> MKPEIEQELSHTLLTELLAYQFASPVRWIETQDVFLKQHNTERIIEIGPSPTLAGMANRTIKAKYESYDAALSLQRQVLCYSKDAKEIYYKPDPADLAPKETPKQEESTPSAPAAATPTPAAAAAPTPAPAPASAGPVESSSGAGSGAGAANSGGAVVDSAALDALTAENKKLAKQQLEVLARYLQVDLNKGSAKSFIKEKEASAVLQKELDLWEAEHGEFYAKGIQPTFSALKSRTYDSYWNWARQDVLSMYFDIIFGKLTSVDRETINQCIQIMNRANPTLIKFMQYHIDHCPEYKGETYKLAKRLGQQLIDNCKQVLTEDPVYKDVSRITGPKTKVSAKGNIEYEETQKDSVRKFEQYVYEMAQGGAMTKVSQPTIQEDLARVYKAISKQASKDSKLELQRVYEDLLKVVESSKEIETEQLTKDILQAATVPTTPTEEVDDPCTPSSDDEIASLPDKTSIIQPVSSTIPSQTIPFLHIQKKTKDGWEYNKKLSSLYLDGLESAAINGLTFKDKYVLVTGAGAGSIGAEILQGLISGGAKVIVTTSRFSKKVTEYYQNMYARYGAAGSTLIVVPFNQGSKQDVDALVQYIYDEPKKGGLGWDLDAIIPFAAIPENGNGLDNIDSKSEFAHRIMLTNLLRLLGAVKSKKTTDTRPAQCILPLSPNHGTFGFDGLYSESKISLETLFNRWYSEDWGSKLTVCGAVIGWTRGTGLMSANNIIAEGIEKLGVRTFSQKEMAFNILGLLTPEIVQLCQEEPVMADLNGGLQFIDNLKDFTSKLRTDLLETADIRRAVSIESAIEQKVVNGDNVDANYSKVMVEPRANMKFDFPTLKSYDEIKQIAPELEGMLDLENVVVVTGFAEVGPWGNSRTRWEMEAYGEFSLEGAIEMAWIMGFIKYHNGNLKGKPYSGWVDAKTQTPIDEKDIKSKYEEEILEHSGIRLIEPELFNGYDPKKKQMIQEVVVQHDLEPFECSKETAEQYKHEHGEKCEIFEIEESGEYTVRILKGATLYVPKALRFDRLVAGQIPTGWDARTYGIPEDTISQVDPITLYVLVATVEALLSAGITDPYEFYKYVHVSEVGNCSGSGMGGVSALRGMFKDRYADKPVQNDILQESFINTMSAWVNMLLLSSSGPIKTPVGACATAVESVDIGIETILSGKAKVVLVGGYDDFQEEGSYEFANMNATSNSIEEFKHGRTPKEMSRPTTTTRNGFMEAQGSGIQVIMTADLALKMGVPIHAVLAMTATATDKIGRSVPAPGKGILTTAREHHGNLKYPSPLLNIEYRKRQLNKRLEQIKSWEETELSYLQEEAELAKEEFGDEFSMHEFLKERTEEVYRESKRQVSDAKKQWGNSFYKSDPRIAPLRGALAAFNLTIDDIGVASFHGTSTVANDKNESATINNMMKHLGRSEGNPVFGVFQKYLTGHPKGAAGAWMLNGAIQILESGLVPGNRNADNVDKLLEQYEYVLYPSRSIQTDGIKAVSVTSFGFGQKGAQAVVVHPDYLFAVLDRSTYEEYATKVSARNKKTYRYMHNAITRNTMFVAKDKAPYSDELEQPVYLDPLARVEENKKKLVFSDKTIQSSQSYVGEVAQKTAKALSTLNKSSKGVGVDVELLSAINIDNETFIERNFTGNEVEYCLNTAHPQASFTGTWSAKEAVFKALGVESKGAGASLIDIEITRDVNGAPKVILHGEAKKAAAKAGVKNVNISISHDDFQATAVALSEF;> MSTHRPFQLTHGSIEHTLLVPNDLFFNYSQLKDEFIKTLPEPTEGFAGDDEPSSPAELYGKFIGFISNAQFPQIVELSLKDFESRFLDNNNDNIHSFAVKLLDDETYPTTIAKVKENIVKNYYKAVKSINKVESNLLYHCKHDAKLVAIFGGQGNTDDYFEELRELYTLYQGLIEDLLVSIAEKLNQLHPSFDKIYTQGLNILSWLKHPETTPDQDYLLSVPVSCPVICVIQLCHYTITCKVLGLTPGEFRNSLKWSTGHSQGLVTAVTIAASDSWDSFLKNSLTAVSLLLFIGSRCLSTYPRTSLPPTMLQDSLDNGEGRPSPMLSVRDLSIKQVEKFIEQTNSHLPREKHIAISLINGARNLVLSGPPESLYGFNLNLRNQKAPMGLDQSRVPFSERKLKCSNRFLPIFAPFHSHLLADATELILDDVKEHGLSFEGLKIPVY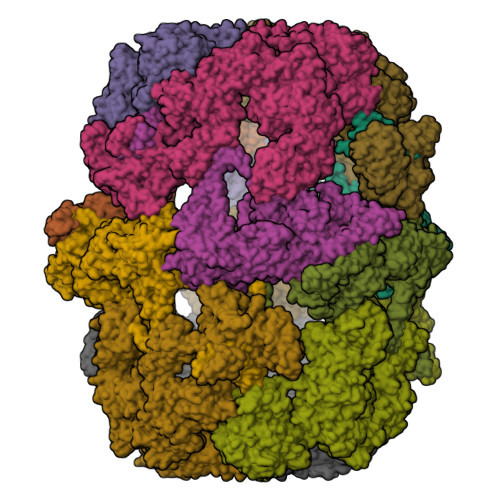DTFDGSDFQALKEPIIDRVVKLITELPVHWEEATNHKATHILDFGPGGVSGLGVLTHRNKEGTGARIILAGTLDSNPIDDEYGFKHEIFQTSADKAIKWAPDWLKELRPTLVKNSEGKIYVKTKFSQLLGRAPLMVAGMTPTTVNTDIVSASLNAGYHIELAGGGYFSPVMMTRAIDDIVSRIKPGYGLGINLIYVNPFMLQWGIPLIKDLREKGYPIQSLTIGAGVPSIEVATEYIEDLGLTHLGLKPGSVDAISQVIAIAKAHPTFPIVLQWTGGRGGGHHSFEDFHQPIIQMYSKIRRCSNIVLVAGSGFGSDEDTYPYLSGYWSEKFNYPPMPFDGVLFGSRVMTSKESHTSLAAKKLIVECKGVPDQQWEQTYKKPTGGIITVRSEMGEPIHKIATRGVMFWKELDDTIFNLPKNKLLDALNKKRDHIIKKLNNDFQKPWFGKNANGVCDLQEMTYKEVANRLVELMYVKKSHRWIDVSLRNMYGDFLRRVEERFTSSAGTVSLLQNFNQLNEPEQFTADFFEKFPQAGKQLISEEDCDYFLMLAARPGQKPVPFVPVLDERFEFFFKKDSLWQSEDLESVVDEDVQRTCILHGPVASQYTSKVDEPIGDILNSIHEGHIARLIKEEYAGDESKIPVVEYFGGKKPASVSATSVNIIDGNQVVYEIDSELPNKQEWLDLLAGTELNWLQAFISTDRIVQGSKHVSNPLHDILTPAKHSKVTIDKKTKKLTAFENIKGDLLPVVEIELVKPNTIQLSLIEHRTADTNPVALPFLYKYNPADGFAPILEIMEDRNERIKEFYWKLWFGSSVPYSNDINVEKAILGDEITISSQTISEFTHAIGNKCDAFVDRPGKATLAPMDFAIVIGWKAIIKAIFPKSVDGDLLKLVHLSNGYKMITGAAPLKKGDVVSTKAEIKAVLNQPSGKLVEVVGTIYREGKPVMEVTSQFLYRGEYNDYCNTFQKVTETPVQVAFKSAKDLAVLRSKEWFHLEKDVQFDVLTFRCESTYKFKSANVYSSIKTTGQVLLELPTKEVIQVGSVDYEAGTSYGNPVTDYLSRNGKTIEESVIFENAIPLSSGEELTSKAPGTNEPYAIVSGDYNPIHVSRVFAAYAKLPGTITHGMYSSASIRALVEEWAANNVAARVRAFKCDFVGMVLPNDTLQTTMEHVGMINGRKIIKVETRNVETELPVLIGEAEIEQPTTTYVFTGQGSQEQGMGMELYNSSEVAREVWDKADRHFVNNYGFSILDIVQNNPNELTIHFGGAKGRAIRDNYIGMMFETIGEDGALKSEKIFKDIDETTTSYTFVSPTGLLSATQFTQPALTLMEKAAYEDIKSKGLIPSDIMFAGHSLGEYSALSSLANVMPIESLVDVVFYRGMTMQVAVPRDELGRSNYGMVAVNPSRVSATFDDSALRFVVDEVANKTKWLLEIVNYNVENQQYVAAGDLRALDTLTNVLNVLKINKIDIVKLQEQMSIEKVKEHLYEIVDEVAAKSLAKPQPIDLERGFAVIPLKGISVPFHSSYLMSGVKPFQRFLCKKIPKSSVKPQDLIGKYIPNLTAKPFELTKEYFQSVYDLTKSEKIKSILDNWEQYE> EEKKEEEKKEEEEKEEEVSEEE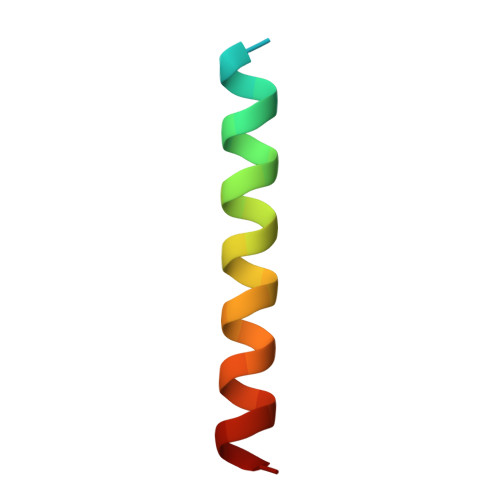ALAGLSALFG> TSWSDRLQNAADMPANMDKHALKKYRREAYHRVFVNRSLAMEKIKCFGFDMDYTLAVYKSPEYESLGFELTVERLVSIGYPQELLSFAYDSTFPTRGLVFDTLYGNLLKVDAYGNLLVCAHGFNFIRGPETREQYPNKFIQRDDTERFYILNTLFNLPETYLLACLVDFFTNCPRYTSCETGFKDGDLFMSYRSMFQDVRDAVDWVHYKGSLKEKTVENLEKYVVKDGKLPLLLSGMKEVGKVFLATNSDYKYTDKIMTYLFDFPHGPKPGSSHRPWQSYFDLILVDARKPLFFGEGTVLRQVDTKTGKLKIGTYTGPLQHGIVYSGGSSDTICDLLGAKGKDILYIGDHIFGDILKSKKRQGWRTFLVIPELAQELHVWTDKSSLFEELQSLDIFLAELYKHLDSSSNERPDISSIQRRIKKVTHDMDMCYGMMGSLFRSGSRQTLFASQVMRYADLYAASFINLLYYPFSYLFRAAHVLM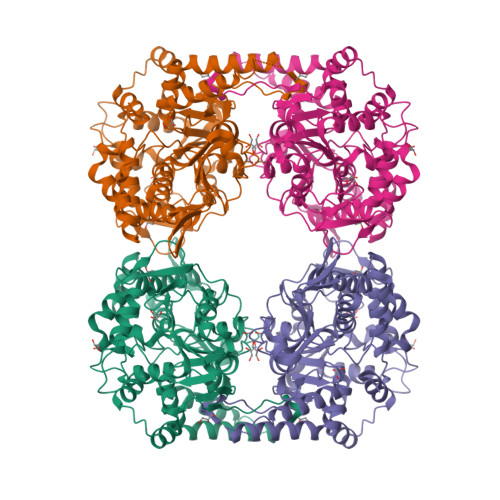PHES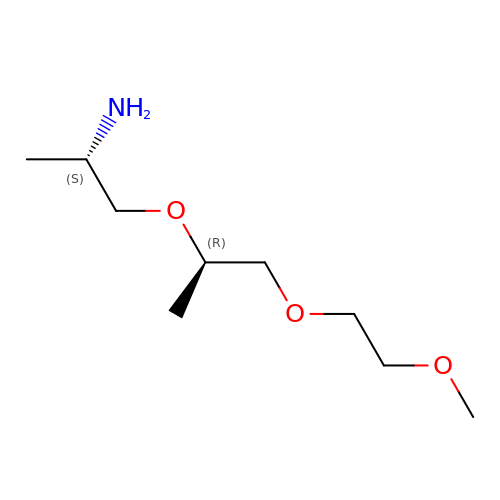(2~{S})-1-[(2~{R})-1-(2-methoxyethoxy)propan-2-yl]oxypropan-2-amine | C9 H21 N O3 | JKCPHDAMWZLSSR-DTWKUNHWSA-N>GSSMSAPTNLEQVLAAGGNTVEMLRNSQIGAYVYPVVAPEFSNWRTEQWAWRNSAVLFDQTHHMVDLYIRGKDALKLLSDTMINSPKGWEPNKAKQYVPVTPYGHVIGDGIIFYLAEEEFVYVGRAPAANWLMYHAQTGGYNVDIVHDDRSPSRPMGKPVQRISWRFQIQGPKAWDVIEKLHGGTLEKLKFFNMAEMNIAGMKIRTLRHGMAGAPGLEIWGPYETQEKARNAILEAGKEFGLIPVGSRAYPSNTLESGWIPSPLPAIYTGDKLKAYREWLPANSYEASGAIGGSFVSSNIEDYYVNPYEIGY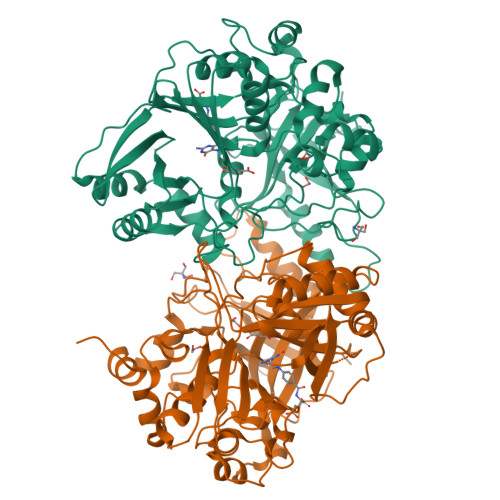GPFVKFDHDFIGRDALEAIDPATQRKKVTLAWNGDDMAKIYASLFDTEADAHYKFFDLPLANYANTNADAVLDAAGNVVGMSMFTGYSYNEKRALSLATIDHEIPVGTELTVLWGEENGGTRKTTVEPHKQMAVRAVVSPVPYSVTARETYEGGWRKAAVTA[2x]> GDDQVSEFKEAFELFDSERTGFITKEGLQTVLKQFGV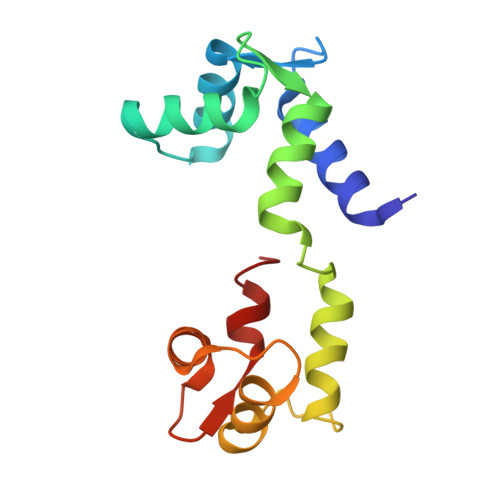RVEPAAFNEMFNEADATGNGKIQFPEFLSMMGRRMKQTTSEDILRQAFRTFDPEGTGYIPKAALQDALLNLGDRLKPHEFAEFLGITETEKGQIRYDNFINTMFT>MRDPTQFEERHLKFLQQLGKGNFGSVEMCRYDPLQDNTGEVVAVKKLQHSTEEHLRDFEREIEILKSLQHDNIVKYKGVCYS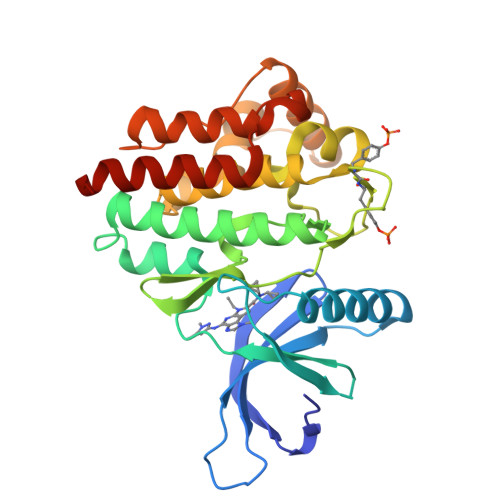AGRRNLKLIMEYLPYGSLRDYLQKHKERIDHIKLLQYTSQICKGMEYLGTKRYIHRDLATRNILVENENRVKIGDFGLTKVLPQDKEYYKVKEPGESPIFWYAPESLTESKFSVASDVWSFGVVLYELFTYIEKSKSPPAEFMRMIGNDKQGQMIVFHLIELLKNNGRLPRPDGCPDEIYMIMTECWNNNVNQRPSFRDLALRVDQIRDNMAGHHHHHH[2x]> PDQFRAIIESPEGAGHVGYQYRRNTGSTMRMVS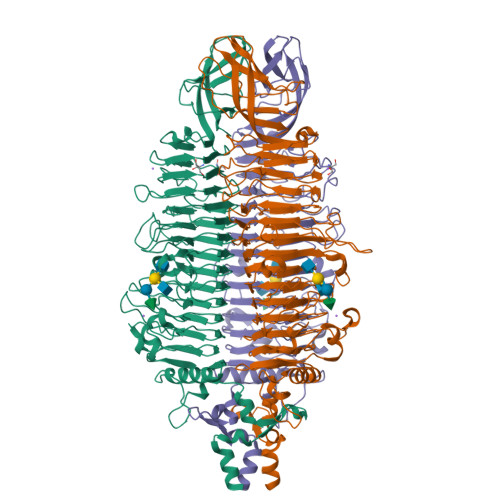DVLDERVSLWDFHCDPSGNVIQPGPNVDSRQYLQAAIDYVSSNGGGTITIPAGYTWYLGSYGVGGIAGHSGIIQLRSNVNLNIEGRIHLSPFFDLKPFQVFVGFDNGDPASSGNLENCHIYGHGVVDFGGYEFGASSQLRNGVAFGRSYNCSVTGITFQNGDVTWAITLGWNGYGSNCYVRKCRFINLVNSSVNAAHSTVYVNCPYSGVESCYFSMSSSFARNIACSVALHQHDTFYRGSTVNGYCRGAYVVMHAAEAAGAGSYAYNMQVENNIAVIYGQFVILGSDVTATVSGHLNDVIVSGNIVSIGERAAFSAPFGAFIDIGPDNSGASNVQDIQRVLVTGNSFYAPANITDSAAITLRANLNGCTFIANNFDCRYMVYNAPGTTSPVVQNLVWDKSNVIGGTHANQRAGQNLFDMQFASVVNSTIEVQLSCEDLSMFSCILFPASCQLSYSKITVDSAWTKSMSNTAVFEGNQQAGANVYVSYPATVNLTSYNTQGAVPFFSTDTNYAWVTSAYSLSINENLDFSPPATYTNKANGQLVGVGYNEIGGVRSVSVRLMLQRQV>[2x]MNTVSPAKKKVIIIGAGIAGLKAA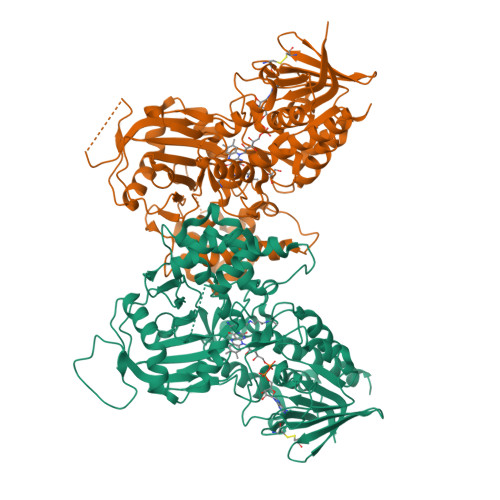STLHQNGIQDCLVLEARDRVGGRLQTVTGYQGRKYDIGASWHHDTLTNPLFLEEAQLSLNDGRTRFVFDDDNFIYIDEERGRVDHDKELLLEIVDNEMSKFAELEFHQHLGVSDCSFFQLVMKYLLQRRQFLTNDQIRYLPQLCRYLELWHGLDWKLLSAKDTYFGHQGRNAFALNYDSVVQRIAQSFPQNWLKLSCEVKSITREPSKNVTVNCEDGTVYNADYVIITVPQSVLNLSVQPEKNLRGRIEFQPPLKPVIQDAFDKIHFGALGKVIFEFEECCWSNESSKIVTLANSTNEFVEIVRNAENLDELDSMLEREDSQKHTSVTCWSQPLFFVNLSKSTGVASFMMLMQAPLTNHIESIREDKERLFSFFQPVLNKIMKCLDSEDVIDGMRPIENIANANKPVLRNIIVSNWTRDPYSRGAYSACFPGDDPVDMVVAMSNGQDSRIRFAGEHTIMDGAGCAYGAWESGRREATRISDLLKLEHHHHHH>ETGRGCPTHCHCEPDGRMLLRVDCSDLGLSELPSNLSVFTSYLDLSMNNISQLLPNPLPSLRFLEELRLAGNALTYIPKGAFTGLYSLKVLMLQNNQLRHVPTEALQNLRSLQSLRLDANHISYVPPSCFSGLHSLRHLWLDDNALTEIPVQAFRSLSALQAMTLALNKIHHIPDYAFGNLSSLVVLHLHNNRIHSLGKKCFDGLHSLETLDLNYNNLDEFPTAIRTLSNLKELGFHSNNIRSIPEKAFVGNPSLITIHFYDNPIQFVGRSAFQHLPELRTLTLNGASQITEFPDLTGTANLESLTLTGAQISSLPQTVCNQLPNLQVLDLSYNLLEDLPSFSVCQKLQKIDLRHNEIYEIKVDTFQQLLSLRSLNLAWNKIAIIHPNAFSTLPSLIKLDLSSNLLSSFPITGLHGLTHLKLTGNHALQSLISSENFPELKVIEMPYAYQCCAFGVCENNGNNGDSVQCSPSGTHHHHHHHHH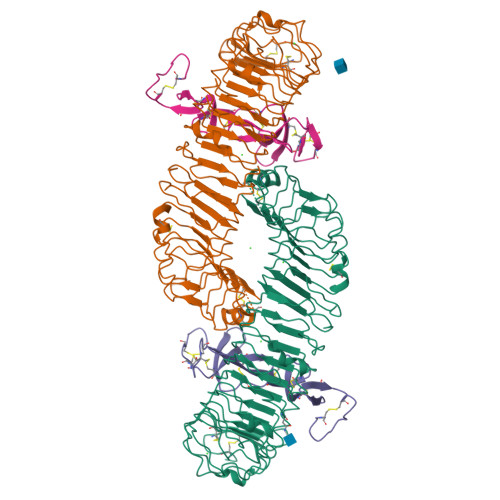H[2x];>ETGICKGCLSCSKDNGCSRCQQKLFFFLRREGMRQYGECLHSCPSGYYGHRAPDMNRCARCRIENCDSCFSKDFCTKCKVGFYLHRGRCFDECPDGFAPLDETMECVEGTHHHHHHHHHH[2x]L-LEUCYL-HYDROXYLAMINE | C6 H14 N2 O2 | 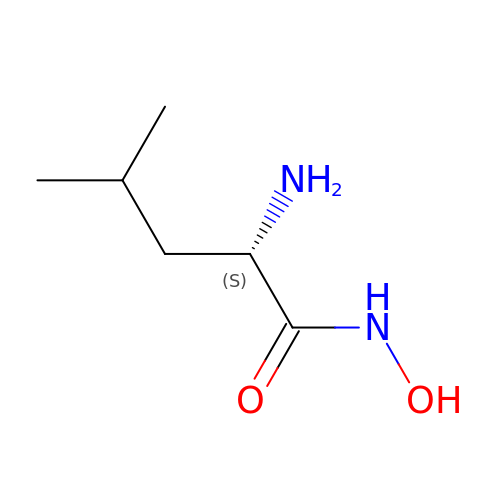UJJHPFLWSVFLBE-YFKPBYRVSA-N>[2x]SNIERNTKLTIDWNSALYHKIRPQDYKNIIETDQGLLIAEIFPKISESSKTPRSLNFALNNLKPILYELIRAHERFSYRHIINNICPKSDTFYSSPKSVIKLLIVCVRKTFPLDLLGSNS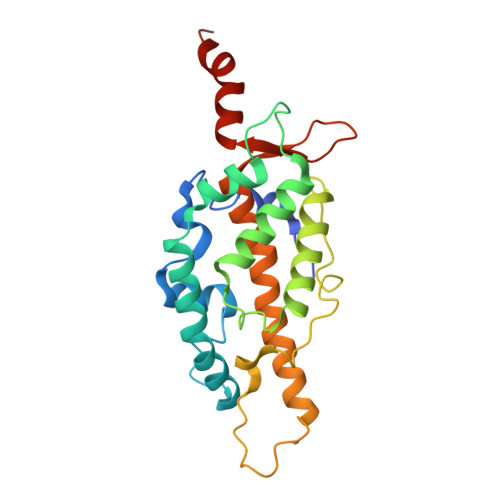NYSVLSKAIAILVKKPLHSKILFDELCKGLRVKDVKWLETRRLPAGEQTQKIPYYDVKNRQALLYKLFFWILSCYVPKLLSTFFYVTELSSTVDIVYIRHDTWKTMSQPFLKSYFRR N1,N14-BIS((S-METHYL)ISOTHIOUREIDO)TETRADECANE | C18 H38 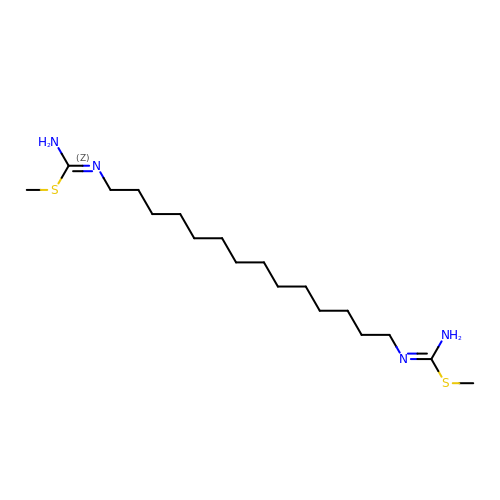N4 S2 | IOKDMHHZKWLWKO-UHFFFAOYSA-N Our focus here is on KAT-II, which is a biologically active homodimer, and reportedly produces almost 75% of KYNA in human brain. The KATs irreversibly convert l-kynurenine (l-KYN), the main intermediate of the kynurenine pathway into KYNA, an endogenous neuroactive agent in CNS, as part of the main route of the tryptophan degradation pathway. KAT-II consists of 425 amino acid residues with its catalytic site at the homodimeric interface. PLP acts as a coenzyme and is covalently linked to Lys263 by a “Schiff base” reaction, resulting in an aldimine linkage.

In this paper the native structure of hKAT-II (PLP form) at 1.83 Å has been determined and refined, providing the highest resolution structure reported. The crystals belonged to the novel tetragonal space group P43212 with unit cell dimensions of a = 102.46 Å, b = 102.46 Å and c = 86.24 Å (α, β and γ = 90°). The asymmetric unit contains one molecule with an estimated solvent content of 48.1%. The final model contains all the residues of a total of 425, containing the one modified residue, LLP (lysine-pyridoxal-5′-phosphate (LLP), which is substituted for Lys263), and 438 solvent molecules. The state in which the side chain amino group of Lys263 forms an aldimine bond with PLP, also referred to as the resting state is the state of the hKAT-II observed with no ambiguity in the electron density maps. Also the N-terminal arm is observed rolled into the location away from the active site, which does not otherwise affect the active site pocket. The oxygen of the pyridine ring hydroxyl moiety of LLP interacts with Asn202 and Tyr233, and the pyridine ring is also sitting parallel to and alongside the Tyr142 ring. Additionally, the pyridoxal ring of LLP has a hydrophobic interaction with Pro232, not previously reported in the other available aminotransferase structures. The side chain carboxylate oxygen of Asp230 takes part in a hydrogen bond with the NH pyridinium of LLP, which is seen to exist across all fold-type I proteins of the PLP-dependent enzyme family, which is generally considered crucial for enzyme function. The biological dimer is observed faithfully in the crystal structure.

> MNYARFITAASAARNPSPIRTMTDILSRGPKSMISLAGGLPNPNMFPFKTAVITVENGKTIQFGEEMMKRALQYSPSAGIPELLSWLKQLQIKLHNPPTIHYPPSQGQMDLCVTSGSQQGLCKVFEMIINPGDNVLLDEPAYSGTLQSLHPLGCNIINVASDESGIVPDSLRDILSRWKPEDAKNPQKNTPKFLYTVPNGNNPTGNSLTSERKKEIYELARKYDFLIIEDDPYYFLQFNKFRVPTFLSMDVDGRVIRADSFSKIISSGLRIGFLTGPKPLIERVILHIQVSTLHPSTFNQLMISQLLHEWGEEGFMAHVDRVIDFYSNQKDAILAAADKWLTGLAEWHVPAAGMFLWIKVKGINDVKELIEEKAVKMGVLMLPGNAFYVDSSAPSPYLRASFSSASPEQMDVAFQVLAQLIKESL(3-{[3-(2-amino-2-oxoethyl)-1-benzyl-2-ethyl-1H-indol-5-yl]oxy}propyl)phosphonic 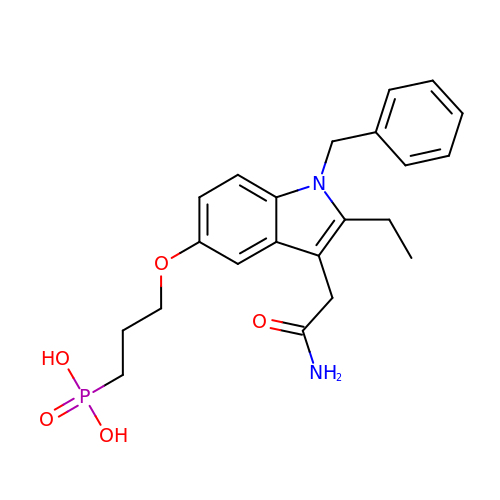acid | C22 H27 N2 O5 P | OPWQYOUZRHDKBR-UHFFFAOYSA-N> MWISIKTLIHHLGVLFFCDYMYNRREKKIIEVKTMRITKVEVDRKKVLISRDKNGGKLVYENEMQDNTEQIMHHKKSSFYKSVVNKTICRPEQKQMKKLVHGLLQENSQEKIKVSDVTKLNISNFLNHRFKKSLYYFPENSPDKSEEYRIEINLSQLLEDSLKKQQGTFICWESFSKDMELYINWAENYISSKTKLIKKSIRNNRIQSTESRSGQLMDRYMKDILNKNKPFDIQSVSEKYQLEKLTSALKATFKEAKKNDKEINYKLKSTLQNHERQIIEELKENSELNQFNIEIRKHLETYFPIKKTNRKVGDIR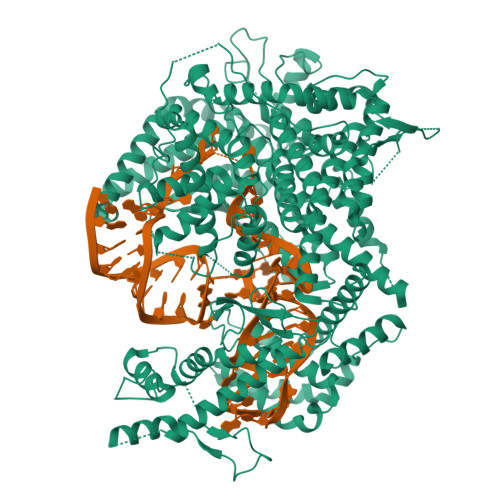NLEIGEIQKIVNHRLKNKIVQRILQEGKLASYEIESTVNSNSLQKIKIEEAFALKFINACLFASNNLRNMVYPVCKKDILMIGEFKNSFKEIKHKKFIRQWSQFFSQEITVDDIELASWGLRGAIAPIRNEIIHLKKHSWKKFFNNPTFKVKKSKIINGKTKDVTSEFLYKETLFKDYFYSELDSVPELIINKMESSKILDYYSSDQLNQVFTIPNFELSLLTSAVPFAPSFKRVYLKGFDYQNQDEAQPDYNLKLNIYNEKAFNSEAFQAQYSLFKMVYYQVFLPQFTTNNDLFKSSVDFILTLNKERKGYAKAFQDIRKMNKDEKPSEYMSYIQSQLMLYQKKQEEKEKINHFEKFINQVFIKGFNSFIEKNRLTYICHPTKNTVPENDNIEIPFHTDMDDSNIAFWLMCKLLDAKQLSELRNEMIKFSCSLQSTEEISTFTKAREVIGLALLNGEKGCNDWKELFDDKEAWKKNMSLYVSEELLQSLPYTQEDGQTPVINRSIDLVKKYGTETILEKLFSSSDDYKVSAKDIAKLHEYDVTEKIAQQESLHKQWIEKPGLARDSAWTKKYQNVINDISNYQWAKTKVELTQVRHLHQLTIDLLSRLAGYMSIADRDFQFSSNYILERENSEYRVTSWILLSENKNKNKYNDYELYNLKNASIKVSSKNDPQLKVDLKQLRLTLEYLELFDNRLKEKRNNISHFNYLNGQLGNSILELFDDARDVLSYDRKLKNAVSKSLKEILSSHGMEVTFKPLYQTNHHLKIDKLQPKKIHHLGEKSTVSSNQVSNEYCQLVRTLLTMK>GSHNLACPTPKEDGLAQQQTQLNLRSLLVNPEGPTLMRLNSVQSSERPLFLVHPIEGSTTVFHSLASRLSIPTYGLQCTRAAPLDSIHSLAAYYIDCIRQVQPEGPYRVAGYSYGACVAFEMCSQLQAQQSPAPTHNSLFLFDGSPTYVLAYTQSYRAKLTPGCEAEAETEAICFFVQQFTDMEHNRVLEALLPLKGLEERVAAAVDLIIKSHQGLDRQELSFAARSFYYKLRAAEQYTPKAKYHGNVMLLRAKTGGAYGEDLGADYNLSQVCDGKVSVHVIEGDHRTLLEGSGLESIISIIHS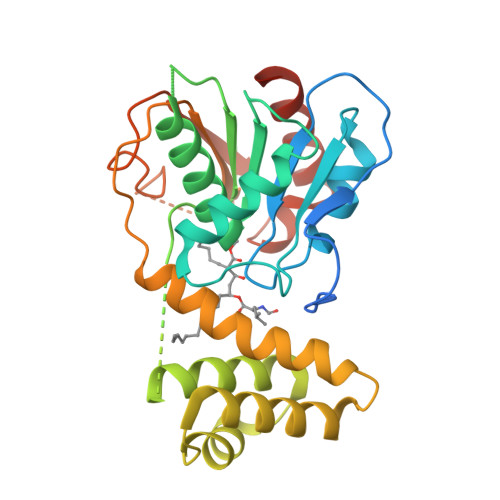SLAEPRVSVREG[2x]> DYPAALQILMEGGTHMVCTGRTHTDRICRFKWLCYSNEAEEFIFFHGNTSVMLPNLGSRRFQPALLDLSTVEDHNTQYFNFVELPAAALRFMPKPVFVPDVALIANRFNPDNLMHVFHDDLLPLFYTLRQFPGLAHEARLFFMEGWGEGAHFDLYKLLSPKQPLLRAQLKTLGRLLCFSHAFVGLSKITTWYQYGFVQPQGPKANILVSGNEIRQFARFMTEKLNASHTGVPLAAEYILVFSRTQNRLILNEAELLLALAQEFQMKTVTVSLEDHTFADVVRLVSNASMLVSMHGAQLVTTLFLPRGATVVELFPYAVNPDHYTPYKTLAMLPGMDLQYVAWRNMMPENTVTHPERPWDQGGITHLDAAEQAAILQSREVPRHLCCRNPEWLFRIYQDTKVDIPSLIQTIRRVVKGAAPRKQAAAAGLYPGKVREARCQASVHGASEARLTVSWQIPWNLKYLKVAEVKYEVWLQEAGEAAYVPYILALQNHTFTENIKPFTTYL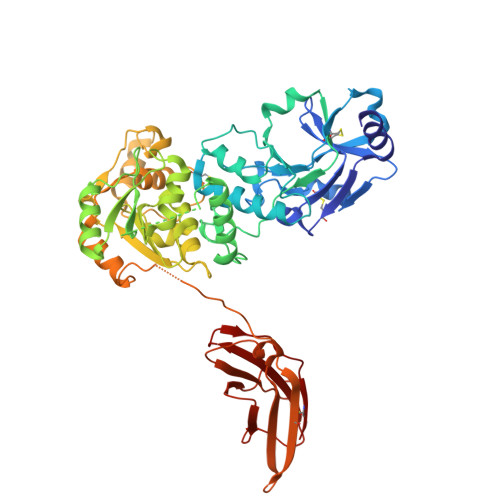VWVRCIFNKILLGPFADVLVCNT> MVLFFEILLVAAVLVITWFAVYA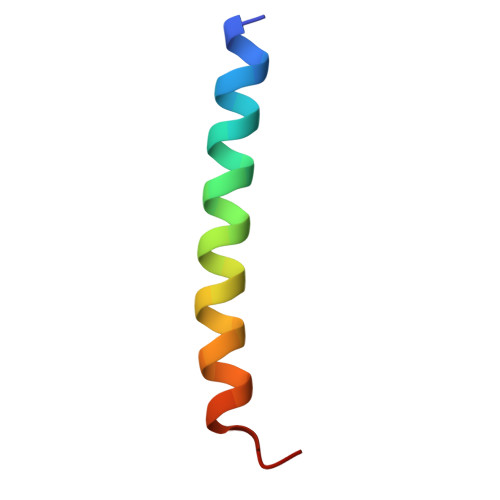LYRLVTDES>[6x]PIELLPETPSQTAGPYVHIGLALEAAGNPTRDQEIWNRLAKPDAPGEHILLLGQVYDGNGHLVRDSFLEVWQADANGEYQ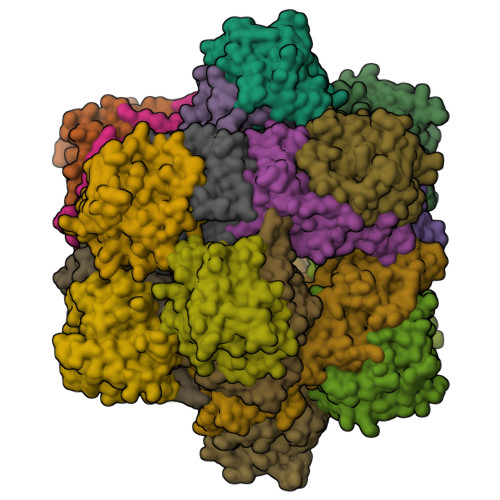DAYNLENAFNSFGRTATTFDAGEWTLHTVKPGVVNNAAGVPMAPHINISLFARGINIHLHTRLYFDDEAQANAKCPVLNLIEQPQRRETLIAKRCEVDGKTAYRFDIRIQGEGETVFFDF;>PAQDNSRFVIRDRNWHPKALTPDYKTSIARSPRQALVSIPQSISETTGPNFSHLGFGAHDHDLLLNFNNGGLPIGERIIVAGRVVDQYGKPVPNTLVEMWQANAGGRCRHKNDRYLAPLDPNFGGVGRCLTDSDGYYSFRTIKPGPYPWRNGPNDWRPAHIHFGISGPSIATKLITQLYFEGDPLIPMCPIVKSIANPEAVQQLIAKLDMNNANPMDCLAYRFDIVLRGQRKTHFENC[6x]Reactions 1 and 4 are catalyzed by two Fe2+-dependent dioxygenases: TML dioxygenase (TMLD) and γ-butyrobetaine dioxygenase (BBD), which are related by homology; reaction 3 is catalyzed by trimethylamino butyraldehyde dehydrogenase (TMABADH); reaction 2, the aldol cleavage of HTML to generate glycine and TMABA, is catalyzed by HTMLA. However, a mouse protein absent in humans (threonine aldolase; Tha1) catalyzes the reaction more efficiently. However, the preferred substrate of Tha1 is HTML with a catalytic efficiency in the order of 104 s−1 M−1, followed by L-allo-threonine (102 s−1 M−1) and L-threonine (101 s−1 M−1). As we found that the mouse enzyme has a strong preference (1000 folds) for HTML towards threonine, the name hydroxytrimethyllysine aldolase (Htmla) would be a better descriptor of the mouse gene.

To verify if the results of our screening for Tha1 are confirmed or improved with the availability of an experimental structure, we decided to determine the crystal structure of mouse Tha1. Mouse Tha1 crystallizes in two space groups, in orthorhombic F222 and in monoclinic C2, with one molecule and two molecules in the ASU, respectively. The PLP cofactor is visible only in the monoclinic structure; however, the active site is very similar in the two cases, with only minor differences. In Tha1, the PLP cofactor, bound to Lys242, is stabilized in the active site by a network of hydrogen bonds and salt bridges with the side chains of Asp211, Arg214 and Thr98 from the same unit, and of Lys267 and Arg274 from the adjacent unit. His123 is making an aromatic stacking interaction with the PLP pyridine ring with a relative distance between the rings of 3.7 Å. The expected tetrameric quaternary structure is formed by crystallographic symmetries, with four identical units in F222 (related by a 222 symmetry) and two identical dimers in C2 (related by a two-fold axis). The RMSD values between the single units (around 0.26–0.28 Å) indicate that the monoclinic and orthorhombic structures are similar. As indicate by data from PISA analysis, the interface between units A and B (analogous to that between units C and D, termed “main interface”) is contributing stronger to the stability of the quaternary structure in comparison with the interface between units A and C (analogous to that between units B and D, termed “secondary interface”). Hence, the tetramer can be considered a dimer (AB + CD) of dimers (A + B and C + D), with the first dissociation being ABCD to AB + CD (as determined by PISA). As a consequence, the tetrameric assembly of the mouse enzyme has a lower stability, with a ΔGdiss (the free energy of assembly dissociation) value of 5–6 kcal/mol compared to the 40.9 kcal/mol of the bacterial enzyme (for the ABCD to AB + CD dissociation).

>[2x]MGSSHHHHHHSSGENLYFQGHMVDLRSDTVTRPGPAMRRAMAEAVVGDDDYGEDPTVHELQEKAAELLGVERTLFVPTNTMANLISVMGHCRRRGSQVLLGQECHLHVYEQGGVAQIAGVHSHPLPDLPYGTLDLNELERALTRGSGSPYHPVCELVYLENTHSSAGGRVLPVDYLRQVCLLAHAHGARVHMDGARLMNAAVALRIPPARLVEHCDSVSFCFSKGLGAPVGALVGGSKDFIGEAWRLRKALGGGMRQAGVLAAAALVGLAEAEEVLPRDHENAQRFAKGLQDLASPICSVDPATVETNMVLVQVAGLPPSELCQRLQAVSAEEVAQTGRAVRVLLFPWTEQSVRAVWHRDVSAQDTELALKKWEFVLRQLRP The facultative intracellular pathogen Listeria monocytogenes, like many related Firmicutes, uses the nucleotide second messenger cyclic di-AMP (c-di-AMP) to adapt to changes in nutrient availability, osmotic stress, and the presence of cell wall-acting antibiotics. cbpB encodes a 150-amino-acid protein that is conserved in some Firmicutes. We determined the structures of free CbpB and CbpB in complex with c-di-AMP at 1.6- and 2.4-Å resolution, respectively. These structures reveal that CbpB has tandem CBS domains (CBS1 and CBS2) that interact to form a disk-like head-to-head homodimer. However, here we found that CbpB is a direct activator of RelA and that c-di-AMP inhibits CbpB-dependent RelA activation.

The structure of free CbpB is similar to the c-di-AMP complex, with root mean square (RMS) distance of 0.86 Å between their equivalent Cα atoms. The major differences between the two structures are within the c-di-AMP binding site. Notably, the conformation of the Tyr45 side chain in free CbpB has severe clashes with the bound position of c-di-AMP, and therefore the binding site does not exist in free CbpB. While these structural differences exist, they do not provide obvious explanations for how CbpB-RelA interactions might be regulated. The CbpB structure exhibits very little change upon c-di-AMP binding and appears as a homodimer in both the free and nucleotide-bound forms, similar to the crystal structure of the CbpB homolog from B. subtilis, DarB (PDB1YAV). It remains unclear how such modest structural changes result in such large impacts on protein-protein interactions, and future work should compare these structural characteristics with those of a CbpB-RelA complex. The third category maps to the conserved surface of CbpB, which is far away from the c-di-AMP binding site and could be involved in another function. Although this analysis is not conclusive, it suggests that this region could be important for the interaction with RelA.

>MGSSHHHHHHSSGMISNRFGQFIDNELADSMISAEKVAHVQLGNNLEHALLVLTKCGYSVIPVLDFEFKLHGLISAAMITDAILGLERIEFERLEDLKVEDVMQTDFPVIKDFNNNERIVHLLVDHPFVCVVDSDHHFEGIVTRRVVLKQVNRYIHLQVEENR[2x]Here we show that the major OMP of the bacterial predator Bdellovibrio bacteriovorus, PopA, differs from this architecture, forming a pentameric porin-like superstructure. The pentameric assembly is radially organized around loop 8, a folded-over edge of the barrel, making a chamber at the centre of the oligomer. The pentamer has a central chamber formed by the association of five loop 8 peptides that is open to the periplasmic side of the bilayer; the chamber is effectively shaped to the dimensions of a lipid monolayer.

Having observed our original structural information from refolded PopA, we set out to interrogate the native folded state, using our existing structure to inform on introducing an internal His-tag in loop 2, referred to hereafter as PopAhis. The protein was successfully solubilized in 1% (w/v) DDM, and was amenable to cryo-EM analysis. A final particle set of 365,835 was subjected to ab initio reconstitution followed by non-uniform refinement in C1 symmetry. The resultant map at 2.85 Å resolution (according to the gold-standard Fourier shell correlation curve with a threshold of 0.143) allowed building of a model with correlation coefficient (CC mask) of 0.87. The cryo-EM structure of PopAhis retains the five-fold arrangement of the X-ray models, demonstrating that differences in native:refolding methodology and DDM:βOG usage have no significant outcome on the PopA structure (chain rmsd to X-ray ranging from 0.7–1.1 Å). The central chamber in PopAhis also has density for alkyl chains, equivalent to 11 DDM molecules, two per monomer with an additional one at the centre. The cryo-EM structure also retains density behind the helix of loop 2, and we were able to validate the x-ray and cryo-EM attribution of this to palmitate (and thus potential FadL-like role) by demonstrating high contact residency time for this ligand during simulations. The density maps from both the x-ray and cryo-EM suggest tight packing of eleven alkyl chains (the central “extra” chain having less defined density in the x-ray map), with chain:chain distances of 4.5 Å commensurate with a crystalline monolayer.

>[5x]SKARVEALANSRHVLDFQTAFDRPYQFMALSEQATIEWGNTGDANPHAEGGFVKRHGDDSAFGAYFGRRSADFSEAVQTVRDASSHHHHHHGSSNPAFADLMFEQNGLNLFYASKMGEWTWGVTAKYSNGKNEDPTVGTKATSAGVAVAASNGTWDFELVQGFTGKSELDNGTVTAEVESKGLTNVTVGYHMSPEMEVYGNVKMSKVEADLNGTPIEVETTSYKVGMVNTLAKSEEGNFFYGVEVASTKVKDDSESLLLPVYMGVEHNAASWLVLRASVAQNVILNETKDDATGNKTDEDSTRMAAGAGIKFGKSVIDASFAGSTTGVINANNLFSQVAYTYTF> GIDPFTSSGGPRKDPIILIPSAASSILTVANIKQFLLESKY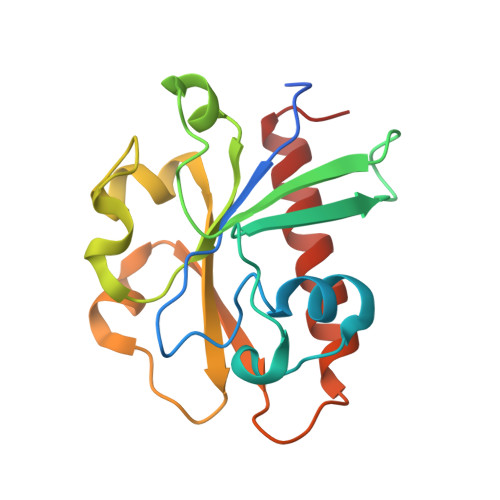VNPRNLPSVPNGLVNIEKNFERISRPIRFIIVDNTRMFTKPEYWDRVVAIFTTGHTWQFNNYQWNSPQELFQRCKGYYFHFAGDSVPQHVQQWNVEKVELDKNKRFKDVEVVRYFWHSLEKELISRGYR>MGNKNTPLNSGKHPDLKIEVAIIGAGTSGLYTAYRLVTDKKFKAHDVQIFDMNNKLGGRLESVIMPGMNFWGELGGMRYLTSQQIVTTLIEGYPLSEKDPNKRTPVLKDKMTPVPFPMGDPSKLLMYLRKERFKQNAWNEAQKKGEKLPTRYYLNENDLGFSSDQLFNKIIYDVLMADPWVAETYGSKIIKGSSVYDYSFKLTSRDWDDIKPKLVYNFPNSPYDQRKVNDIGFWNLIKDQVSQEGYEFLANAGGYYSNTINWNSAEAFPYMVGDFSAGTIYKTIEEGYDSIAYAVANSYMEHEGACIWSENKLLTFTK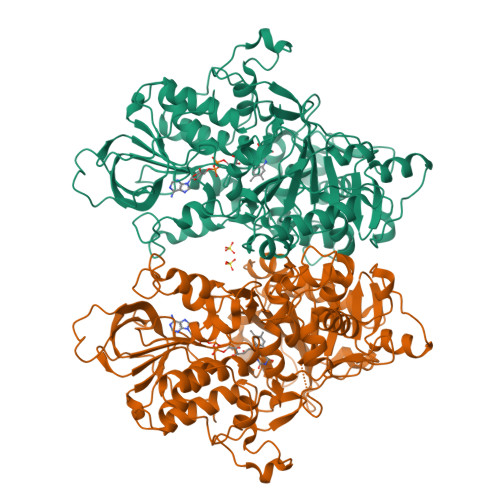DHPLTNTHKYELTFLNLKTNTQWKVYANSIVLAMPRKSLELLDQNNFFFNINKNSVLNNNIRSVIMEPAFKILMGFEYPWWKELGIDSGHSITDLPMRQCYYFGTDPETNNSMLLGSYGDMETETFWKALSDDKVLFEVKAAKSASLRELHQLDDVQATKLMVGELMNQLRELHGDTVTIPEPYVTYFKDWTDEPFGAGYHAWKAGFSVENVMPYMRKPLTDEQIHICGEAYSDQQGWVEGAFCEAEKMLQEYFGLDRPYWLSPDYYLGWEHHHHHH[2x]> MNEKNIKHSQNFITSKHNIDKIMTNIRLNEHDNIFEIGSGKGHFTLELVQRCNFVTAIEIDHKLCKTTENKLVDHDNFQVLNKDILQFKFPKNQSYKIFGNIPYNISTDIIRKIVFDSIADEIYLIVEYGFAKRLLNTKRSLALFLMAEVDISILSMVPREYFHPKPKVNS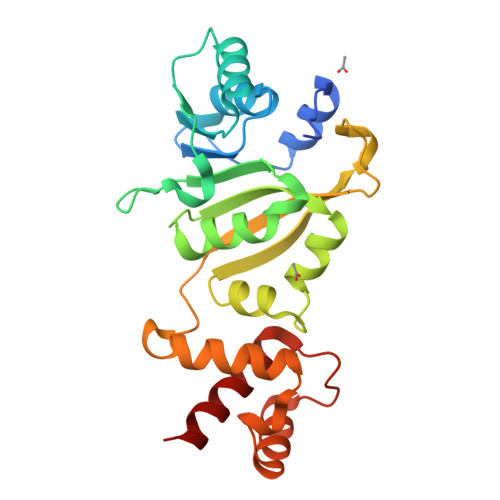SLIRLNRKKSRISHKDKQKYNYFVMKWVNKEYKKIFTKNQFNNSLKHAGIDDLNNISFEQFLSLFNSYKLFNK>[4x]ALFTGIIPPVSTIFTADGQLDKPGTAALIDDLIKAGVDGLFFLGSGGEFSQLGAEERKAIARFAIDHVDRRVPVLIGTGGTNARETIELSQHAQQAGADGIVVINPYYWKVSEANLIRYFEQ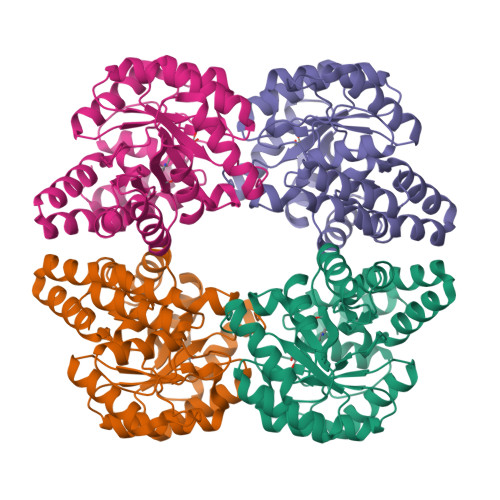VADSVTLPVMLYNFPALTGQDLTPALVKTLADSRSNIIGIKDTIDSVAHLRSMIHTVKGAHPHFTVLCGYDDHLFNTLLLGGDGAISASGNFAPQVSVNLLKAWRDGDVAKAAGYHQTLLQIPQMYQLDTPFVNVIKEAIVLCGRPVSTHVLPPASPLDEPRKAQLKTLLQQLKLC>[8x]GSSHHHHHHSSGLVPGGSHMVSKGEENNMAVIKPDMKIKLRMEGAVNGHPFAIEGVGLGKPFEGKQSMDLKVKEGGPLPFAYDILTTVFCYGNRVFAKYPENIVDYFKQSFPEGYSWERSMNYEDGGICNATNDITLDGDCYIYEIRFDGVNFPANGPVMQKRTVKWEPSTEKLYVRDGVLKGDVNQALSLEGGGHYRCDFKTTYKAKKVVQLPDYHFVDHHIEIKSHDKDYSNVNLHEHAEAHSG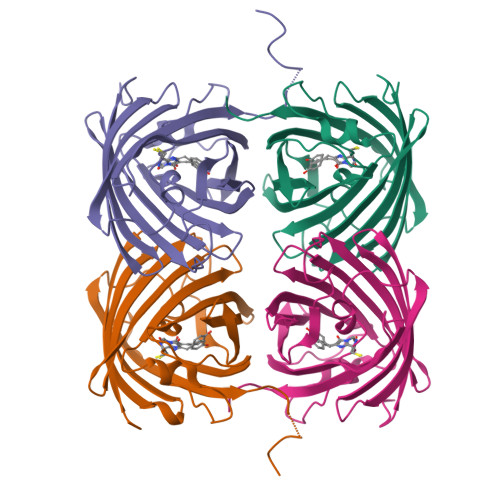LPRQAMDELYK>GHMSAAEPHYIDAQRAIAPVDAPLAAPHEYAAVLRSDFVSSYHDGRDVWTDEAAMRPASAILHAHLGRPAVVLDAGAGRGRDTAYFLEQGHRVTAVDLVEPPEWAPLAQRWGERVRFVACPVSELDGEARFDGALDNGCLHHQHPDAYGTYLARIHALLRPDGRFTISVFESDGPGRLYANHAQRLYREFTEPELAE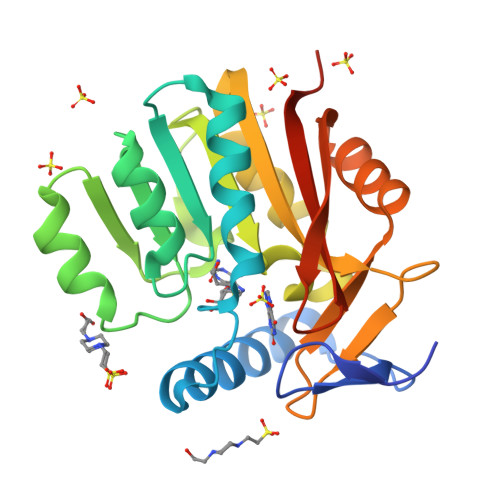LLRAAHFTPVDSQRVPRPKAGLHYLVMTARKTDSTDASGRR[2x]>[2x]TPEMPVLENRAAQGNITAPGGARRLTGDQTAALRNSLSDKPAKNIILLIGDGMGDSEITAARNYAEGAGGFFKGIDALPLTGQYTHYALNKKTGKPDYVTDSAASATAWSTGVKTYNGALGVDIHEKDHPTILEMAKAAGLATGNVSTAELQDATPAALVAHVTSRKCYGPSATSQ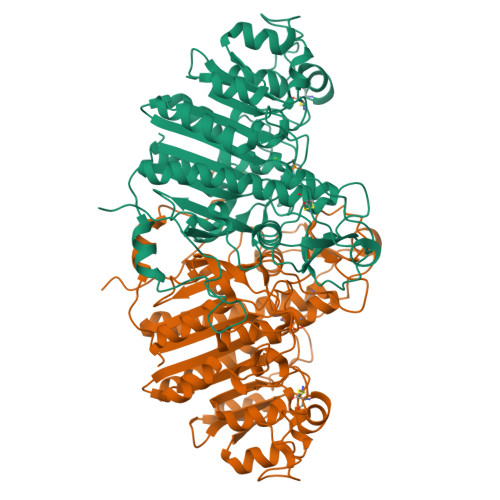KCPGNALEKGGKGSITEQLLNARADVTLGGGAKTFAETATAGEWQGKTLREEAEARGYQLVSDAASLNSVTEANQQKPLLGLFADGNMPVRWLGPKATYHGNIDKPAVTCTPNPQRNDSVPTLAQMTDKAIELLSKNEKGFFLQVEGASIDKQDHAANPCGQIGETVDLDEAVQRALEFAKKEGNTLVIVTADHAHASQIVAPDTKAPGLTQALNTKDGAVMVMSYGNSEEDSQEHTGSQLRIAAYGPHAANVVGLTDQTDLFYTMKAALGLK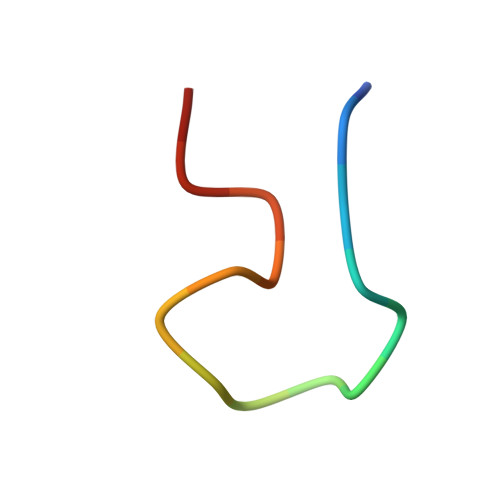> GASDGSGWSSENNPWG N-[(3S)-2-oxotetrahydrofuran-3-yl]butanamide | C8 H13 N O3 | 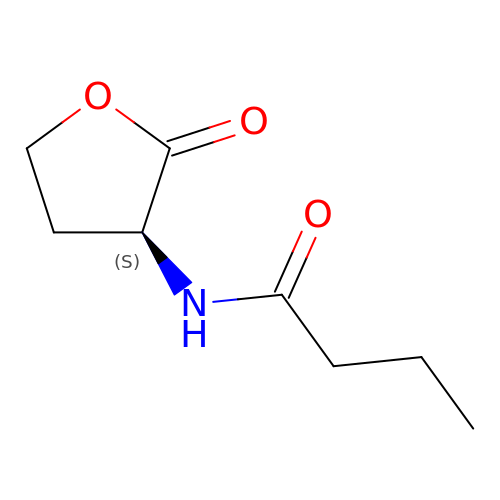VFFNZZXXTGXBOG-LURJTMIESA-N The major regulator of virulence factors in L. monocytogenes is the transcription activator PrfA, a member of the Crp/Fnr family of regulators. PrfAWT is a homodimer in which each monomer consists of an N-terminal domain (residues 1 to 108) and a C-terminal DNA-binding domain (residues 138 to 237) linked by a long α-helix (αC, residues 109 to 137). Two α-helices in the C-terminal domain, αE (residues 170 to 178) and αF (residues 183 to 197), constitute the two helices of the typical HTH motif present in many prokaryotic transcription factors. Glutathione binding stabilizes the DNA-binding helix-turn-helix (HTH) motif in a conformation compatible with DNA-binding, thereby allowing expression of PrfA-regulated virulence factors.

In addition, we found three new PrfA mutants in the remaining three strains—Leu to His substitution at residue 140 (PrfAL140H), Ala to Gly substitution at residue 218 (PrfAA218G), and Ala to Val substitution at residue 94 (PrfAA94V). All the previously identified PrfA* mutants, i.e., PrfAG145S, PrfAG145C, and PrfAL140F, could grow in this medium with G-6-P, as could the PrfA mutants PrfAL140H and PrfAA218G, whereas the strain carrying the PrfAA94V mutation was unable to grow. The PrfAG145S, PrfAG145C, and PrfAL140F mutants showed the highest expression levels, followed by PrfAA218G and PrfAL140H. To gain a deeper understanding of the PrfA* mutant proteins, the crystal structures of purified PrfAL140H, PrfAL140F, and PrfAA218G were determined as individual proteins and in complex with the PrfA hly promoter DNA. We expected that the crystal structures of PrfAL140H, PrfAL140F, and PrfAA218G would be similar to the PrfAG145S structure, since our in vivo characterization classified them as PrfA* mutations. However, their structures showed that each of the PrfA* variants had only one folded HTH motif, with the remaining structure residing in the PrfAWT conformation. The PrfAL140H, PrfAL140F, and PrfAA218G PrfA* mutants all had a folded HTH motif in one monomer of the homodimer but an uncollapsed central core structure. Consequently, we suggest that these mutant structures represent an intermediately activated form of the protein with features characteristic of both inactive and activated PrfA. The most striking structural difference between the inactive, intermediate-active, and fully active structures is the position of their recognition helices. When superimposed on monomer B, the recognition helix in monomer A is shifted up to 6 Å.

>[2x]GAMNAQAEEFKKYLETNGIKPKQFHKKELIFNQWDPQEYCIFLYDGITKLTSISENGTIMNLQYYKGAFVIMSGFIDTETSVGYYNLEVISEQATAYVIKINELKELLSKNLTHFFYVFQTLQKQVSYSLAKFNDFSINGKHGSICGQLLILTYVYGKETPDGIKITLDNLTMQELGYSSGIAHSSAVSRIISKLKQEKVIVYKNSCFYVQNLDYLKRYAPKLDEWFYLACPATWGKLN>GSHMTTPSHLSDRYELGEILGFGGMSEVHLARDLRDHRDVAVKVLRADLARDPSFYLRFRREAQNAAALNHPAIVAVYDTGEAETPAGPLPYIVMEYVDGVTLRDIVHTEGPMTPKRAIEVIADACQALNFSHQNGIIHRDVKPANILISATNAVKVVDFGIARAIADSGNSVTQTAAVI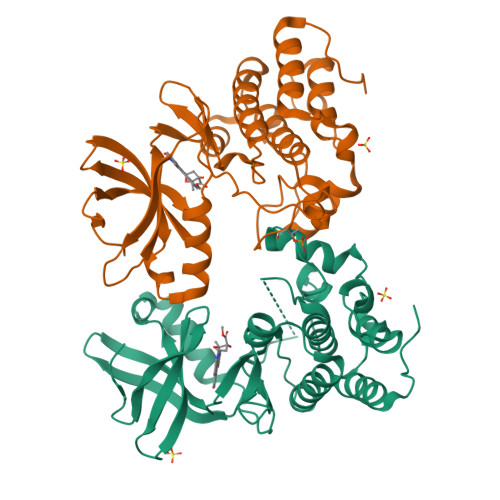GTAQYLSPEQARGDSVDARSDVYSLGCVLYEVLTGEPPFTGDSPVSVAYQHVREDPIPPSARHEGLSADLDAVVLKALAKNPENRYQTAAEMRADLVRVHNGEPPEAPKVLTDAERTSLLSSAAGNLSGPR[2x]>GAGEARLEEAVNRWVLKFYFHEALRAFRGSRYGDFRQIRDIMQALLVRPLGKEHTVSRLLRVMQCLSRIEEGENLDCSFDMEAELTPLESAINVLEMIKTEFTLTEAVVESSRKLVKEAAVIICIKNKEFEKASKILKKHMSKDPTTQKLRNDLLNIIREKNLAHPVIQNFSYETFQQKMLRFLESHLDDAEPYL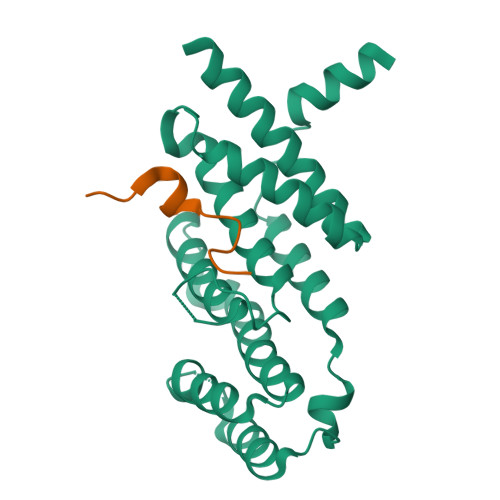LTMAKKALK[2x];>SQETFEEKYRLSPTLSSTKGH[2x]> HEEGNDVRRNFDVSKISGYWYSVLLASDVREKTEENSSMRVF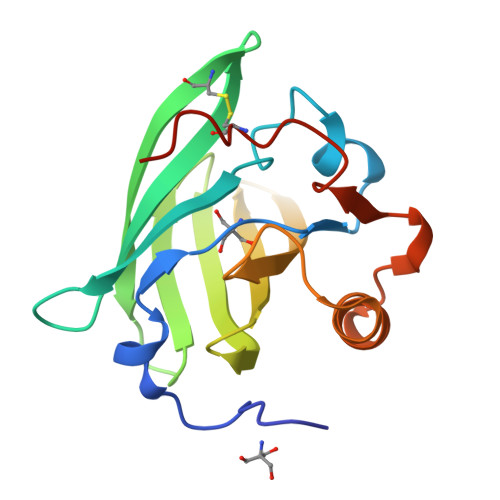VNHIEVLSNSSLLFNMHIKVDGKCTEIALVSDKTEKDGEYSVEYDGYNVFRIVETDYTDYIIFHLVNFKEKDSFQMMELSAREPDTSEEVRKRFVEYCQKHGIVKENIFDLTEVDRCLQARGSEKA> MLCHNRLLLVNKQTQKYRTKLRYRFRQPSVVPLRQTLQQRHNTILEVLRRRRINSGDQSP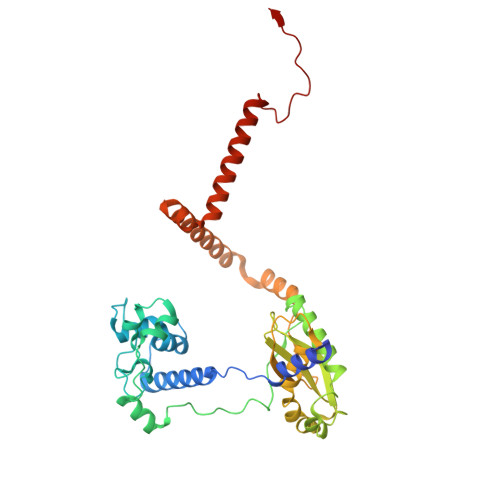YRYVEERLYSKPSRLDREGVKVNKTYALQGLGDLEPLRYGANFGISEKDALKYETVAEKAKYMEPPIPYSSLAARKLAAGALWPAAPDPEGMISKEVRLLRHESSMSPSARAFSERVAYHLRRSLKACPGHIAEHIDFTQLIIQEVLGSRRSKEIYIVWFTVDPGARFELEPRLHQLNHWVQQLIIKRVKRRPHIPRVTWIYDGGRLERELPRDVKQELQSFVADAATTLESRVKYLKELDTMNQRMKDIPWFMPYLWSKEEKAARQKSMLADLEEVERRKNEHSSGRSAPPRTSPPPQFVR To compensate for this, archaea, prokaryotes and eukaryotes have photolyase proteins, which repair damaged DNA using the energy of visible light. The photoreceptor protein uses near-UV and visible light (300–500 nm) as an energy source to monomerize (6–4)TT [or (6–4)CC] lesions in DNA.

The room-temperature structure was solved to 2.27 Å resolution and was obtained by serial femtosecond crystallography (SFX) using an X-ray free-electron laser. For SFX experiments, we developed a batch crystallization protocol in combination with a seeding method and successfully produced crystals with a homogeneous size distribution of 20–40 µm. Using only 975 µg of protein, we recorded 209 242 diffraction images with a total acquisition time of about 2 h. Indeed, the mean r.m.s.d. calculated on the main-chain residues is 0.35 Å, which indicates that the position of the main chains was unchanged. However, some of the positions of the side chains change at the higher temperature. The residues with high r.m.s.d. values for side chains are located either on surface regions or loop regions. The X-ray pulses at free-electron lasers are so short that diffraction is recorded before absorbed X-rays can do damage to the protein structure, and we therefore presume that our SFX structure is not subject to radiation damage. In our SFX structure the isoalloxazine atoms occupy the same plane, and butterfly bending along the N5–N10 plane was not observed. Despite their small size, our microcrystals diffracted beyond 2.27 Å, a resolution that is high enough to be able to observe conformational changes of side chains upon blue-light activation and is suitable for a time-resolved pump–probe serial crystallographic experiment.

> DSQRSTLVHWFRKGLRLHDNPALSHIFTAANAAPGRYFVRPIFILDPGILDWMQVGANRWRFLQQTLEDLDNQLRKLNSRLFVVRGKPAEVFPRIFKSWRVEMLTFETDIEPYSVTRDAAVQKLAKAEGVRVETHCSHTIYNPELVIAKNLGKAPITYQKFLGIVEQLKVPKVLGVPEKLKNMPTPPKDEVEQKDSAAYDCPTMKQLVKRPEELGPNKFPGGETEALRRMEESLKDEIWVARFEKPNTAPNSLEPSTTVLSPYLKFGCLSARLFNQKLKEIIKRQPKHSQPPVSLIGQLMWREFYYTVAAAEPNFDRMLGNVYCMQIPWQEHPDHLEAWTHGRTGYPFIDAIMRQLRQEGWIHHLARHAVACFLTRGDLWISWEEGQRVFEQLLLDQDWALNAGNWMWLSASAFFHQYFRVYSPVAFGKKTDPQGHYIRKYVPELSKYPAGCIYEPWKASLVDQRAYGCVLGTDYPHRIVKHEVVHKENIKRMGAAYKVNRE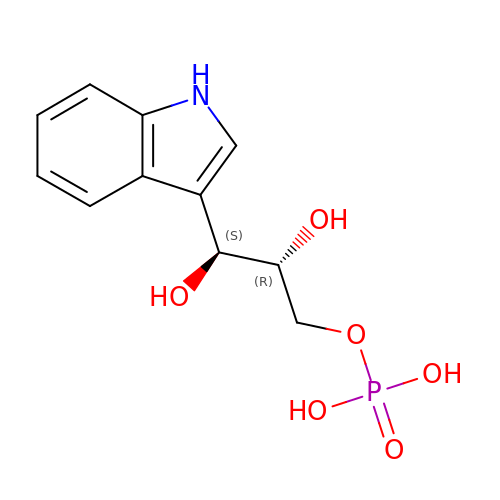INDOLE-3-GLYCEROL PHOSPHATE | C11 H14 N O6 P | NQEQTYPJSIEPHW-MNOVXSKESA-N>ATQTGATWGLDRIDQRTLPLSGTFTYSNTGSGVNAYIIDTGIRVSHSEFGGRATAVFDAIGDGQNGNDCNGHGTHVAGTVGGTVYGVAKSVRLYAVRVLNCSGSGSNSGVIAGVDWVRQNARRPAVANMSLGGGASSALDTAVNNAINAGITFALAAGNSNRDACQFSPARVTAGITVGATTSTDARASYSNYGSCLDLFAPGSSITSAWISSDTSTNTISGTSMATPHVAGVAALYLQSNPSASPATVRNAIVGNAT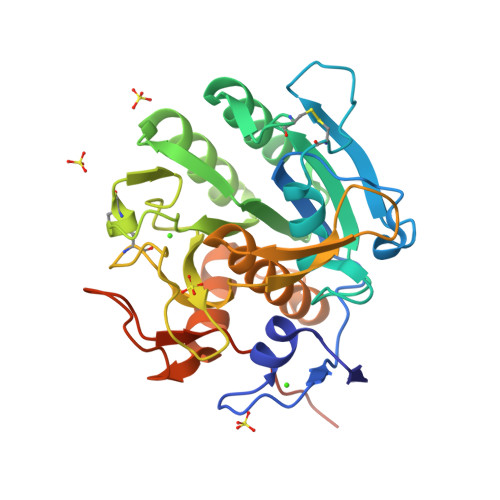SGVVSNAGRRSPNLLLYSNYENLYFQSHHHHHHWSHPQFEK[3x]> GDVEEAIERAVVHVADTMRSGPSNSASVPALTAVETGHTSQVTPSDTMQTRHVKNYHSRSESTVENFLGRSACVYMEEYKTTDNDVNKKFVAWPINTKQMVQMRRKLEMFTYLRFDMEVTFVITSRQDPGTTLAQDMPVLTHQIMYVPPGGPIPAKVDDYAWQTSTNPSIFWTEGNAPARMSIPFISIGNAYSNFYDGWSNFDQRGSYGYNTLNNLGHIYVRHVSGSSPHPITSTIRVYFKPKHTRAWVPRPPRLCQYKKAFSVDFTPTPITDTRKDINTVTT;> SPTVEECGYSDRVRSITLGNSTITTQECANVVVGYGRWPTYLRDDEATAEDQPTQPDVATCRFYTLDSIKWEKGSVGWWWKFPEALSDMGLFGQNMQYHYLGRAGYTIHVQCNASKFHQGCLLVVCVPEAEMGGAVVGQAFSATAMANGDKAYEFTSATQSDQTKVQTAIHNAGMGVGVGNLTIYPHQWINLRTNNSATIVMPYINSVPMDNMFRHYNFTLMVIPFVKLDYADTASTYVPITVTVAPMCAEYNGLRLAQAQ;> GLPTMNTPGSTQFLTSDDFQSPCALPQFDVTPSMNIPGEVKNLMEIAEVDSVVPVNNVQDTTDQMEMFRIPVTINAPLQQQVFGLRLQPGLDSVFKHTLLGEILNYYAHWSGSMKLTFVFCGSAMATGKFLIAYSPPGANPPKTRKDAMLGTHIIWDIGLQSSCVLCVPWISQTHYRLVQQDEYTSAGYVTCWYQTGMIVPPGTPNSSSIMCFASACNDFSVRMLRDTPFISQDNKLQ;> GAQVSTQKTGAHETSLSAAGNSIIHYTNI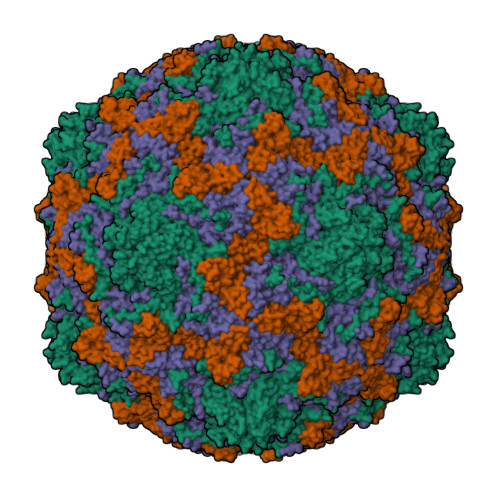NYYKDAASNSANRQDFTQDPSKFTEPVKDVMIKSLPALN> MGSSHHHHHHMRKEIDPETSKYFSEIANLFDSNEVELEERSVICGNALEETRGREYEIATDYIISHVLQTLLEGCELDQLCSFIRNSASVFPAIAMDRSGSHVAESALKSLATHLENPDAYSVIEEALHSICKVIVDNPLDMMCNCYGSHVLRRLLCLCKGVSLDSPELYGAKSSKALAKRLNLKMSQLDDNNLEIPHQGFPGMLTYLLSGLLSCSREDMKYLQVDQYSSLVLQTALRLMLKQDEQLLEIIPLILRCNSTNKKVEGFHIETNVAKEILESMKDNSFSHLVEVILEVAPESLYNEMFNKVFKNSLFELSVDRCANFVIQALISHARDQEQMGIMWEELAPRFKDLL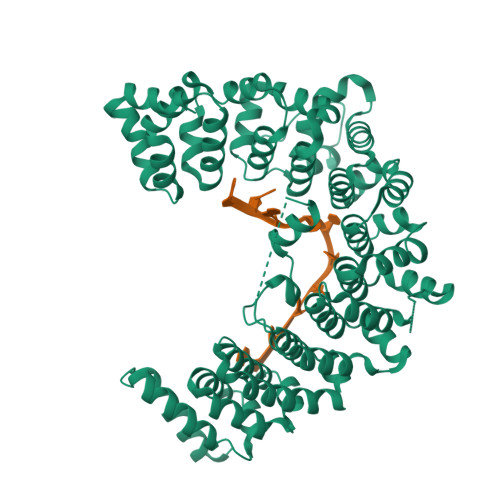EQGKSGVVASLIAVSQRLQSHENKCCEALVGAVCSTNESRISILPRLLFLDYYFGCRDKSTWEWAPGAKMHVMGCLILQGIFKFSSDHIQPYITSLTSMKAEYITETAKDSSGARVIEAFLASDAATKQKRRLIIKLRGHFGELSLHTSGSFTVEKCFDACNLTLREAIASELLDVKVDLSKTKQGPYLLRKLDIDGYASRPDQWKSRQEAKQSTYNEFCSAFGSNK>[2x]MAITADDIAVQYPIPTYRFIVTLGDEQVPFTSASGLDINFDTIEYRDGTGNWFKMPGQRQAPNITLSKGVFPGKNAMYEWINAIQLNQVEKKDIMISLTNEAGTEVLVSWNVSNAFPTSLTSPSFDATSNEIAVQQITLMADRVTIQTA;> MTVTTTYPGVYLSEDAVSSFSVNSAATAVPLFAYDSENTNTINKPIQVFRNWAEFTVEYPTPLEDAFYTSLSLWFMHGGGKCYLVNEANIADAVAQYDDITLIVAAGTDTTTYTAFTTVVGQGYRIFGLFDGPKEKIAGTAKPDEVMEEYPTSPFGAVFYPWGTLASGAAVPPSAIAAASITQTDRTRGVWKAPANQAVNGVTPAFAVSDDFQGKYNQGKALNMIRTFSGQGTVVWGARTLEDSDNWRYIPVRRLFNAVERDIQKSLNKLVFE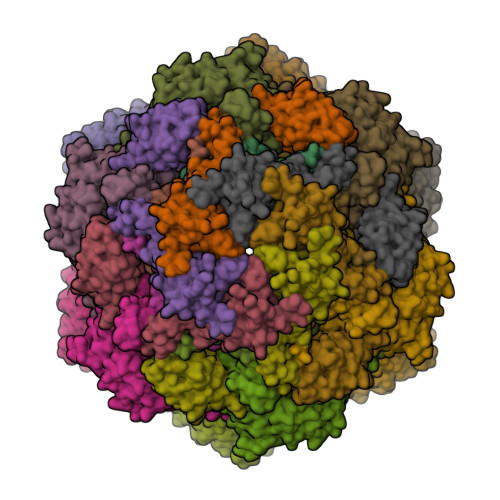PNSQPTWQRVKAAVDSYLHSLWQQGALAGNTPADAWFVQVGKDLTMTQEEINQGKMIIKIGLAAVRPAEFIILQFSQDIAQ;> MATVTSVPGVYIEEDASPAMSVSASATAVPLFVARFTPLKPELAGVITRIGSWLDYTILFDSNVPSSARVTVSSTAVEPSPEFDALETASSKATTTYTYQIDDTEVVDPTASVALRLYFQNGGGPCYLYPLEKADDNGPLAALPDLIDEVGEITLLASPDPDETYRTAVYGALAASLDQHKGYFLLADSVNGDAPSAVGGSAQVAVYYPNVEVPHTRKLDDAEVAIDGYLDDEGKAVTTLAALRVVNTEFAGEIAQSLSGDLSAPLSLPPSALIAGVYGKTDGERGVWKAPANVVLNGVSDVSVRVTNEQQAELNPKGINVIRHFSDRGLVVWGSRTQKDDDDWRYIPVRRLFDAAERDIKKALQPMVFEPNSQLTWKRVQTAIDNYLYRLWQQGALAGNKAEEAYFVRVGKGITMTQDEINQGKMIIQVGMAAVRPAEFIILKFTQDMSQ;> MSMSNYQTLVDVNNAMNKMLRAYVNEAVAIRFDLPDVDATQADAAISVFLYDIHEDLQLRTAESRGFNAGAGRLLPGWVNVKCNYLITYWESTGPATDADNPDSQPDNQAIQVMSQVLAALINNRQLADIPGAYTQVMPPKENLNSLGNFWQSLGNRPRLSLNYCVTVPISLSDKGEEMTPVKSLSTTVEPKAPLSPLVITDALREQLRVALGGDYDACLAMTHVNLDSSPVANSDGSAAEIRVSLRVYGMTPTEYLAPMNTVFNEWEKSEAAAVTPDGYRVYINAVDKTDLTGI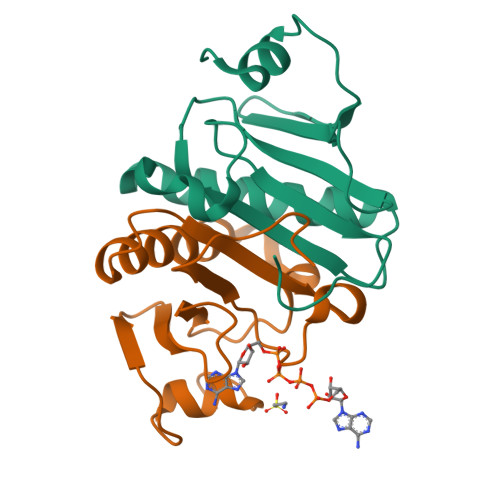>[2x]SLMADEIAKAQVARPGGDTIFGKIIRKEIPAKIIFEDDRCLAFHDISPQAPTHFLVIPKKHISQISVAEDDDESLLGHLMIVGKKCAADLGLNKGYRMVVNEGSDGGQSVYHVHLAVLGGRQMHWPPG3-AMINO-N-{4-[2-(2,6-DIMETHYL-PHENOXY)-ACETYLAMINO]-3-HYDROXY-1-ISOBUTYL-5-PHENYL-PENTYL}-BENZAMIDE 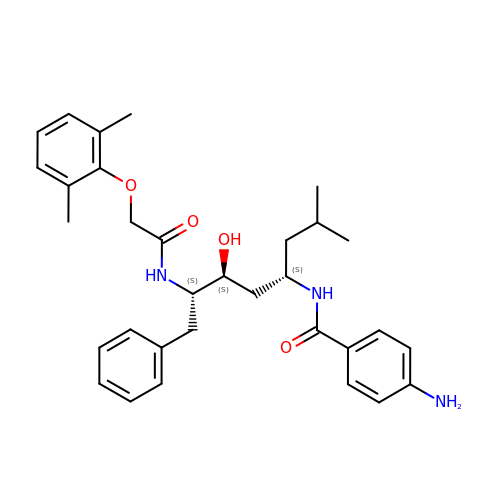| C32 H41 N3 O4 | APJAEXGNDLFGPD-AWCRTANDSA-N> MFNKDQDYWVSVYSTKDFLSVETDSGLGRV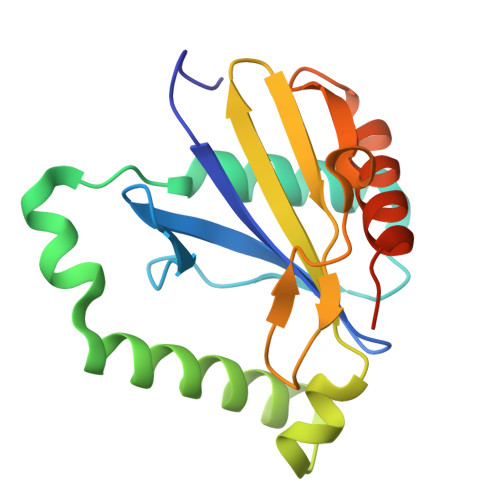RRDPLFPSHLLPPDADNQTIGDAVLIALSNSRTLSLEESADFFDLETGKEQYATWIAMLMEKYGYKTKRALFKDMKNCSIHCINDLITISPTRHEKLEAWSGRGIKESDDVVIPADSIPEEIGAALRLALSRCKGTSLEHHHHHH> MKSSHHHHHHENLYFQSNAALTTISPHDAQELIARGAKLIDIRDADEYLREHIPEADLAPLSVLEQSGLPAKLRHEQIIFHDQAGKRTSNNADKLAAIAAPAEIFLLEDGIDGWKKAGLP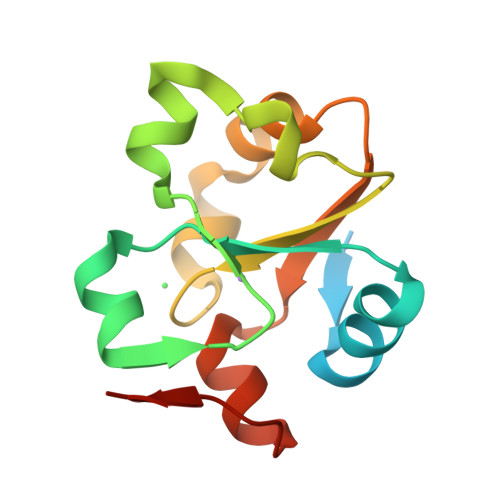VAVNKSQ> GSHMLTKQQIRYCLDEMAKMFPDAHCELVHRNPFELLIAVVLSAQCTDALVNKVTKRLFEKYRTPHDYIAVPLEELEQDIRSIGLYRNKARNIQKLCAMLIDKYNGEVPRDRDELMKLPGVGRKTANVVVSVAFGVPAIAVDTHVERVSKRLGFCRWDDSVLEVEKTLMKIIPKEEWSITHHRMIFFGRYHCKAQSPQCPSCPL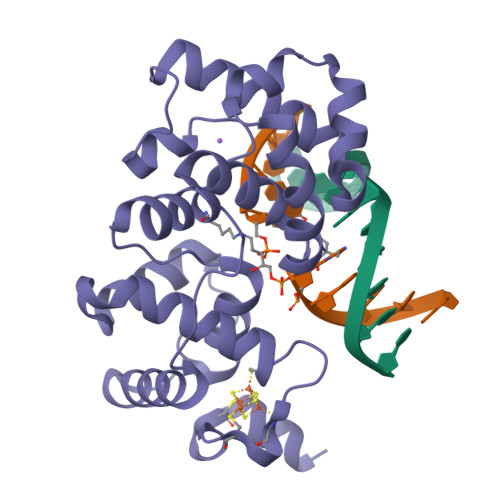LHLCREGKKRMRKREEKAANQK>[3x]GAMGSWNPKYDTRTLWTTPDTSPNCTIAQDKDSKLTLVLTKCGSQILANVSLIVVAGKYHIINNKTNPKIKSFTIKLLFNKNGVLLDNSNLGKAYWNFRSGNSN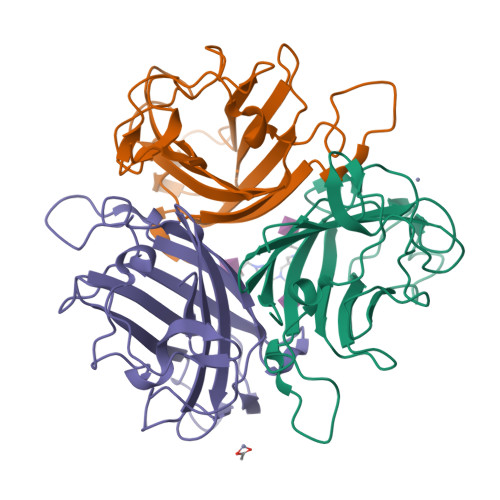VSTAYEKAIGFMPNLVAYPKPSNSKKYARDIVYGTIYLGGKPDQPAVIKTTFNQETGCEYSITFNFSWSKTYENVEFETTSFTFSYIAQE>[4x]MTLQKDKVIKWVRFTPPQVLAIGFFLTIIIGAVLLMLPISTTKPLSWIDALFTAASATTVTGLAVVDTGTQFTVFGQTVIMGLIQIGGLGFMTFAVLIVMILGKKIGLKERMLVQEALNQPTIGGVIGLVKVLFLFSISIELIAALILSIRLVPQYGWSSGLFASLFHAISAFNNAGFSLWPDNLMSYVGDPTVNLVITFLFITGGIGFTVLFDVMKNRRFKTFSLHTKLMLTGTLMLNAIAMLTVFILEYSNPGTLGHLHIVDKLWASYFQAVTPRTAGFNSLDFGSMREGTIV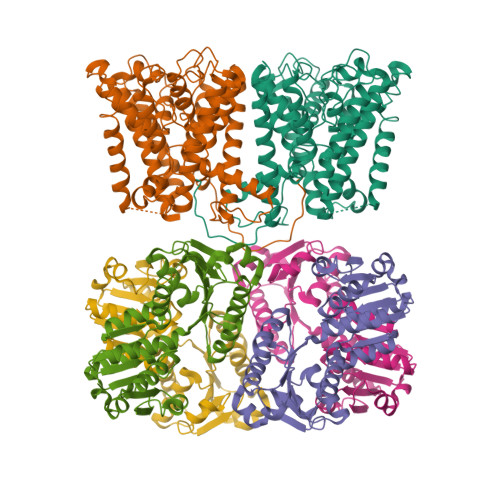FTLLLMFIGAGSASTASGIKLTTFIVILTSVIAYLRGKKETVIFRRSIKYPIIIKALAVSVTSLFIVFLGIFALTITEQAPFLQIVFETFSAFGTVGLTMGLTPELTTAGKCIIIVIMFIGRIGPLTFVFSFAKTEQSNIRYPDGEVFTG;>MGRIKNKQFAVIGLGRFGGSIVKELHRMGHEVLAVDINEEKVNAYASYATHAVIANATEENELLSLGIRNFEYVIVAIGANIQASTLTTLLLKELDIPNIWVKAQNYYHHKVLEKIGADRIIHPEKDMGVKIAQSLSDENVLNYLEGSKQFAVIGLGRFGGSIVKELHRMGHEVLAVDINEEKVNAYASYATHAVIANATEENELLSLGIRNFEYVIVAIGANIQASTLTTLLLKELDIPNIWVKAQNYYHHKVLEKIGADRIIHPEKDMGVKIAQSLSDENLELVPR[4x]>XSLSDKDKAAVRALWSKIGKSADAIGNDALSRMIVVYPQTKTYFSHWPDVTPGSPHIKAHGKKVMGGIALAVSKIDDLKTGLMELSEQHAYKLRVDPANFKILNHCILVVISTMFPKEFTPEAHVSLDKFLSGVALALAERYR[2x];>VEWTDKERSIISDIFSHMDYDDIGPKALSRCLIVYPWTQRHFSGFGNLYNAEAIIGNANVAAHGIKVLHGLDRGVKNMDNIAATYADLSTLHSEKLHVDPDNFKLLSDCITIVLAAKMGHAFTAETQG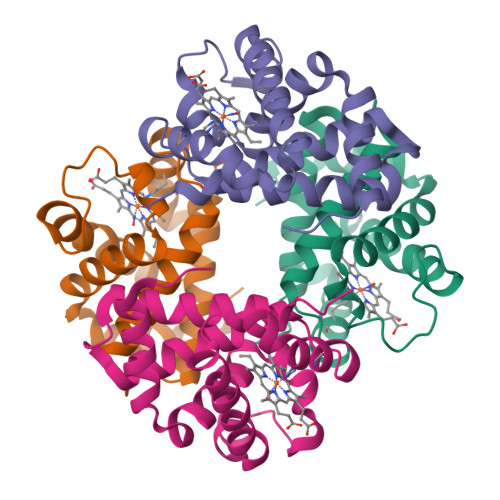AFQKFLAVVVSALGKQYH[2x]>[2x]GSMGAMERVLKVFHYFENSSEPTTWASIIRHGDATDVRGIIQKIVDCHKVKNVACYGLRLSHLQSEEVHWLHLDMGVSNVREKFELAHPPEEWKYELRIRYLPKGFLNQFTEDKPTLNFFYQQVKNDYMLEIADQVDQEIALKLGCLEIRRSYGEMRGNALEKKSNYEVLEKDVGLRRFFPKSLLDSVKAKTLRKLIQQTFRQFANLNREESILKFFEILSPVYRFDKECFKCALGSSWIISV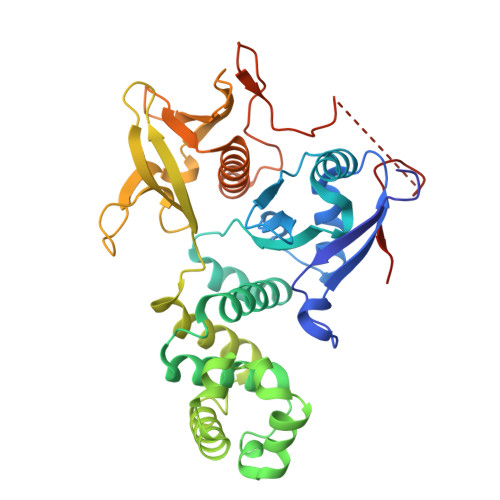ELAIGPEEGISYLTDKGANPTHLADFNQVQTIQYSNSEDKDRKGMLQLKIAGAPEPLTVTAPSLTIAENMADLIDGYCRLVNGATQSFIIRPQKEGERALPSIPKLANNEKQGVRSHTVSVSETDDYAEIIDEED> MPVITVNTNVAEKSIPVFFQAALTNMMTKALQKPKEVMFVDLRSGANIMMGGDRNPCVFATVECIGRLNP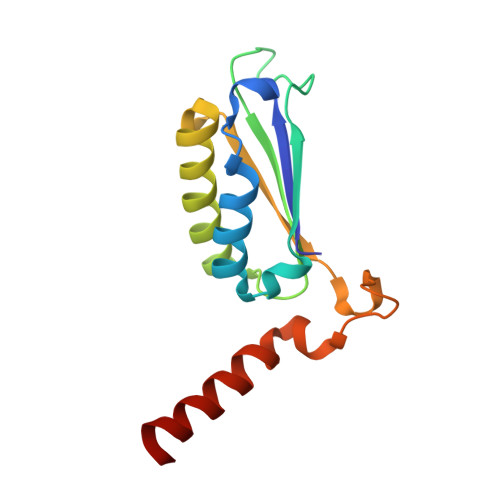TSNLAMARDMEDMFIEHLNVRRERIVIRFIPVPALFCSFNGALHDVSIERDEDIISQAIAEYLHHHHH> MTTTMKISIEFLEPFRMTKWQESTRRNKNNKEFVRGQAFARWHRNKKDNTKGRPYITGTLLRSAVIRSAENLLTLSDGKISEKTCCPGKFDTEDKDRLLQLRQRSTLRWTDKNPCPDNAETYCPFCELLGRSGNDGKKAEKKDWRFRIHFGNLSLPGKPDFDGPKAIGSQRVLNRVDFKSGKAHDFFKAYEVDHTRFPRFEGEITIDNKVSAEARKLLCDSLKFTDRLCGALCVIRFDEYTPAADSGKQTENVQAEPNANLAEKTAEQIISILDDNKKTEYTRLLADAIRSLRRSSKLVAGLPKDHDGKDDHYLWDIGKKKKDENSVTIRQILTTSADTKELKNAGKWREFCEKLGEALYLKSKDMSGGLKITRRILGDAEFHGKPDRLEKSRSVSIGSVLKETVVCGELVAKTPFFFGAIDEDAKQTALQVLLTPDNKYRLPRSAVRGILRRDLQTYFDSPCNAELGGRPCMCKTCRIMRGITVMDARSEYNAPPEIRHRTRINPFTGTVAEGALFNMEVAPEGIVFPFQLRYRGSEDGLPDALKTVLKWWAEGQAFMSGAASTGKGRFRMENAKYETLDLSDENQRNDYLKNWGWRDEKGLEELKKRLNSGLPEPGNYRDPKWHEINVSIEMASPFINGDPIRAAVDKRGTAVVTFVKYKAEGEEAKPVCAYKAESFRGVIRSAVARIHMEDGVPLTELTHSDCECLLCQIFGSEYEAGKIRFEDLVFESDPEPVTFDHVAIDRFTGGAAAKKKFDDSPLPGSPARPLMLKGSFWIRRDVLEDEEYCKALGKALADVNNGLYPLGGKSAIGYGQVKSLGIKGDDKRISRLMNPAFDETDVAVPEKPKTDAEVRIEAEKVYYPHYFVEPHKKVEREEKPCGHQKFHEGRLTGKIRCKLITKTPLIVPDTSNDDFFRPADKEARKEKDEYHKSYAFFRLHKQIMIPGSELRGMVSSVYETVTNSCFRIFDETKRLSWRMDADHQNVLQDFLPGRVTADGKHIQKFSETARVPFYDKTQKHFDILDEQEIAGEKPVRMWVKRFIKRLSLVDPAKHPQKKQDNKWKRRKEGIATFIEQKNGSYYFNVVTNNGCTSFHLWHKPDNFDQEKLEGIQNGEKLDCWVRDSRYQKAFQEIPENDPDGWECKEGYLHVVGPSKVEFSDKKGDVINNFQGTLPSVPNDWKTIRTNDFKNRKRKNEPVFCCEDDKGNYYTMAKYCETFFFDLKENEEYEIPEKARIKYKELLRVYNNNPQAVPESVFQSRVARENV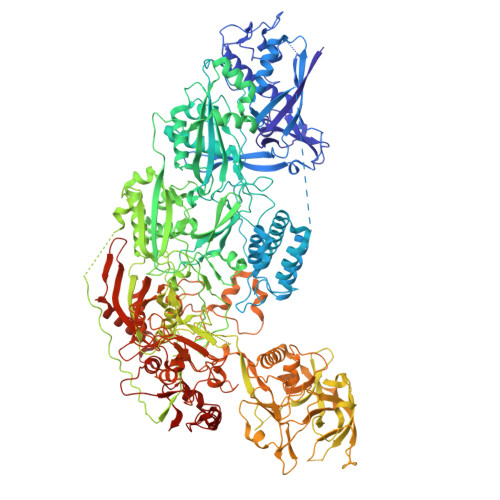EKLKSGDLVYFKHNEKYVEDIVPVRISRTVDDRMIGKRMSADLRPCHGDWVEDGDLSALNAYPEKRLLLRHPKGLCPACRLFGTGSYKGRVRFGFASLENDPEWLIPGKNPGDPFHGGPVMLSLLERPRPTWSIPGSDNKFKVPGRKFYVHHHAWKTIKDGNHPTTGKAIEQSPNNRTVEALAGGNSFSFEIAFENLKEWELGLLIHSLQLEKGLAHKLGMAKSMGFGSVEIDVESVRLRKDWKQWRNGNSEIPNWLGKGFAKLKEWFRDELDFIENLKKLLWFPEGDQAPRVCYPMLRKKDDPNGNSGYEELKDGEFKKEDRQKKLTTPWTPWASSGLVPRGSHHHHHHH>[2x]APSPIIKFPGDVAPKTDKELAVQYLNTFYGCPKESCNLFVLKDTLKKMQKFFGLPQTGDLDQNTIETMRKPRCGNPDVANYNFFPRKPKWDKNQITYRIIGYTPDLDPETVDDAFARAFQVWSDVTPLRFSRIHDGEADIMINFGRWEHGDGYPFDGKDGLLAHAFAPGTGVGGDSHFDDDELWTLGEGQVVRVKYGNADGEYCKFPFLFNGKEYNSCTDTGRSDGFLWCSTTYNFEKDGKYGFCPHEALFTMGGNAEGQPCKFPFRFQGTSYDSCTTEGRTDGYRWCGTTEDYDRDKKYGFCPETAMSTVGGNSEGAPCVFPFTFLGNKYESCTSAGRSDGKMWCATTANYDDDRKWGFCPDQGYSLFLVAAHAFGHAMGLEHSQDPGALMAPIYTYTKNFRLSQDDIKGIQELYGASPDIDLGTGPTPTLGPVTPEICKQDIV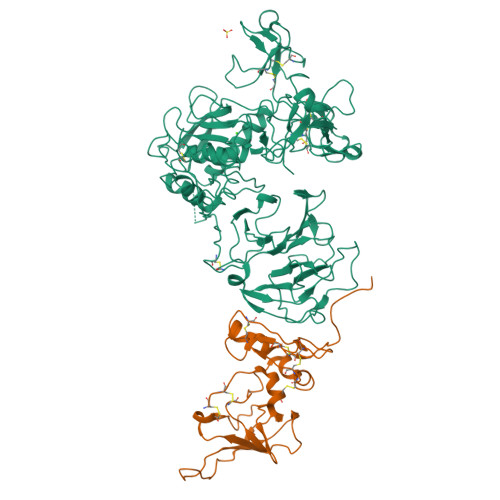FDGIAQIRGEIFFFKDRFIWRTVTPRDKPMGPLLVATFWPELPEKIDAVYEAPQEEKAVFFAGNEYWIYSASTLERGYPKPLTSLGLPPDVQRVDAAFNWSKNKKTYIFAGDKFWRYNEVKKKMDPGFPKLIADAWNAIPDNLDAVVDLQGGGHSYFFKGAYYLKLENQSLKSVKFGSIKSDWLGC;>[2x]CSCSPVHPQQAFCNADVVIRAKAVSEKEVDSGNDIYGNPIKRIQYEIKQIKMFKGPEKDIEFIYTAPSSAVCGVSLDVGGKKEYLIAGKAEGDGKMHITLCDFIVPWDTLSTTQKKSLNHRYQMGCECKITRCPMIPCYISSPDECLWMDWVTEKNINGHQAKFFACIKRSDGSCAWYRGAAPPKQEFLDIEDP> MSWQEKINAALDARRAADALRRRYPVAQGAGRWLVADDRQYLNFSSNDYLGLSHHPQIIR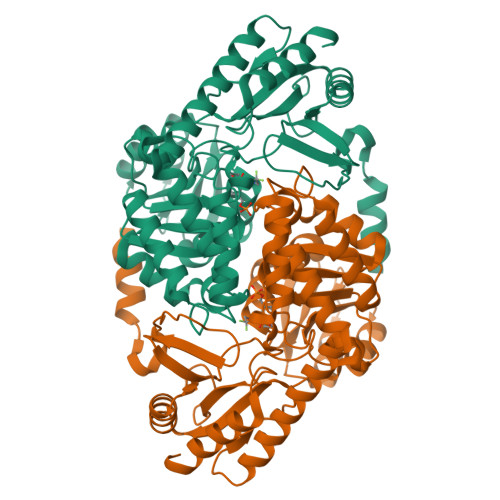AWQQGAEQFGIGSGGSGHVSGYSVVHQALEEELAEWLGYSRALLFISGFAANQAVIAAMMAKEDRIAADRLSHASLLEAASLSPSQLRRFAHNDVTHLARLLASPCPGQQMVVTEGVFSMDGDSAPLAEIQQVTQQHNGWLMVDDAHGTGVIGEQGRGSCWLQKVKPELLVVTFGKGFGVSGAAVLCSSTVADYLLQFARHLIYSTSMPPAQAQALRASLAVIRSDEGDARREKLAALITRFRAGVQDLPFTLADSCSAIQPLIVGDNSRALQLAEKLRQQGCWVTAIRPPTVPAGTARLRLTLTAAHEMQDIDRLLEVLHGNG> MDKVQYLTRSAIRRASTIEMPQQARQALQCLFINFCAILICLLLI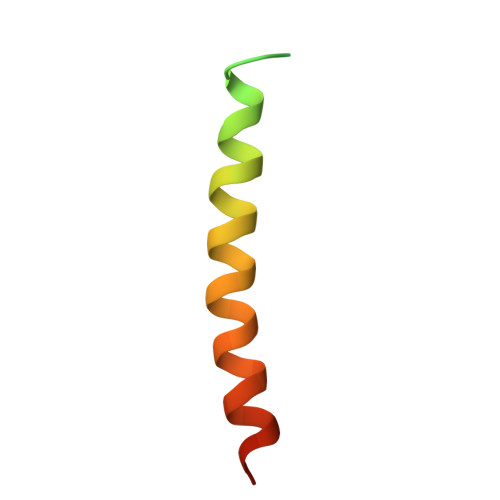CIIGMLL[1-(4-chlorobenzoyl)-5-methoxy-1H-indol-3-yl]acetic 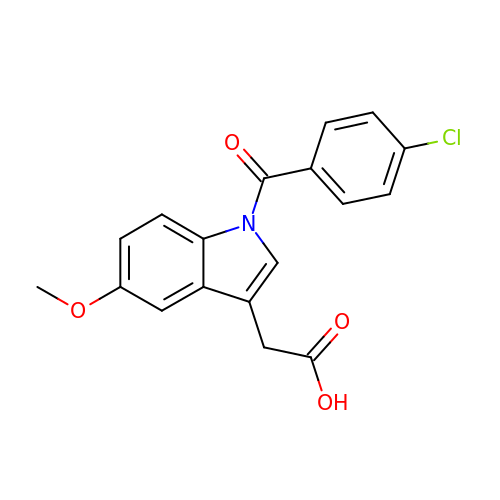acid | C18 H14 Cl N O4 | DHEMTWWLRLOBKI-UHFFFAOYSA-N> G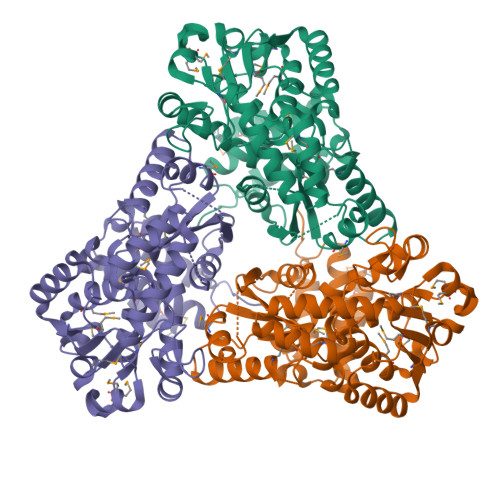SHMMKTVNELIKDINSLTSHLHEKDFLLTWEQTPDELKQVLDVAAALKALRAENISTKVFNSGLGISVFRDNSTRTRFSYASALNLLGLAQQDLDEGKSQIAHGETVRETANMISFCADAIGIRDDMYLGAGNAYMREVGAALDDGYKQGVLPQRPALVNLQCDIDHPTQSMADLAWLREHFGSLENLKGKKIAMTWAYSPSYGKPLSVPQGIIGLMTRFGMDVTLAHPEGYDLIPDVVEVAKNNAKASGGSFRQVTSMEEAFKDADIVYPKSWAPYKVMEERTELLRANDHEGLKALEKQCLAQNAQHKDWHCTEEMMELTRDGEALYMHCLPADISGVSCKEGEVTEGVFEKYRIATYKEASWKPYIIAAMILSRKYAKPGALLEQLLKEAQERVK(5S)-2-amino-3-methyl-5-phenyl-5-[(3S,5S,7S)-tricyclo[3.3.1.1~3,7~]dec-1-yl]-3,5-dihydro-4H-imidazol-4-one | C20 H25 N3 O | 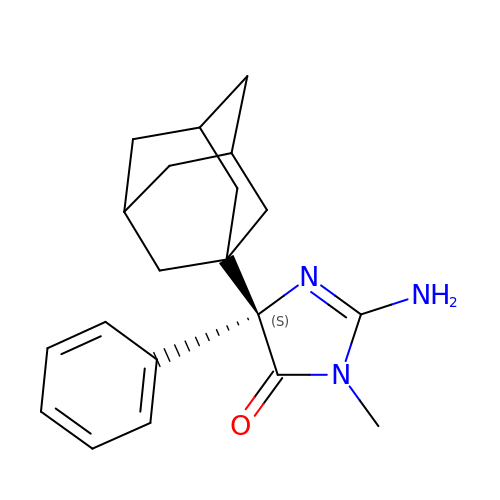BEDDENNXVBITIQ-WYIOCLOVSA-N>[2x]MMSGQGKRLMVMAGGTGGHVFPGLAVAHHLMAQGWQVRWLGTADRMEADLVPKHGIEIDFIRISGLRGKGIKALIAAPLRIFNAWRQARAIMKAYKPDVVLGMGGYVSGPGGLAAWSLGIPVVLHEQNGIAGLTNKWLAKIATKVMQAFPGAFPNAEVVGNPVRTDVLALPLPQQRLAGREGPVRVLVVGGSQGARILNQTMPQVAAKLGDSVT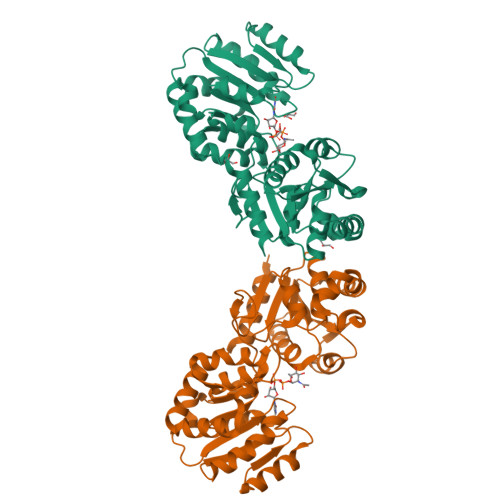IWHQSGKGSQQSVEQAYAEAGQPQHKVTEFIDDMAAAYAWADVVVCRSGALTVSEIAAAGLPALFVPFQHKDRQQYWNALPLEKAGAAKIIEQPQLSVDAVANTLAGWSRETLLTMAERARAASIPDATERVANEVSRVARALEHHHHHH> MGSDSIDTPNYDVQKHINKLCGMLLITED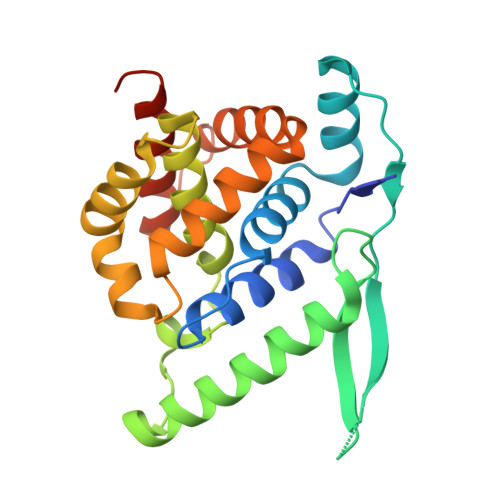ANHKFTGLIGMLYAMSRLGREDTIKILRDAGYHVKANGVDVTTHRQDINGKEMKFEVLTLASLTTEIQINIEIESRKSYKKMLKEMGEVAPEYRHDSPDCGMIILCIAALVITKLAAGDRSGLTAVIRRANNVLKNEMKRYKGLLPKDIANSFYEVFEKHPHFIDVFVHFGIAQSSTRGGSRVEGIFAGLFMNAYGLEHHHHHH>[3x]GPGGAERPTLPIPDLLTTDARNRI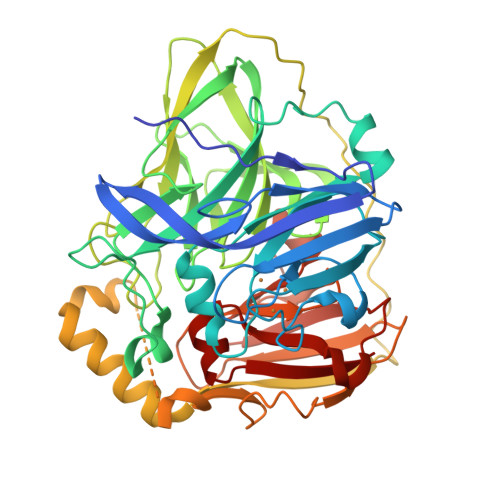QLTIGAGQSTFGGKTATTWGYNGNLLGPAVKLQRGKAVTVDIYNQLTEETTLHWHGLEVPGEVDGGPQGIIPPGGKRSVTLNVDQPAATCWFHPHQHGKTGRQVAMGLAGLVVIEDDEILKLMLPKQWGIDDVPVIVQDKKFSADGQIDYQLDVMTAAVGWFGDTLLTNGAIYPQHAAPRGWLRLRLLNGCNARSLNFATSDNRPLYVIASDGGLLPEPVKVSELPVLMGERFEVLVEVNDNKPFDLVTLPVSQMGMAIAPFDKPHPVMRIQPIAISASGALPDTLSSLPALPSLEGLTVRKLQLSMDPMLDMMGMQMLMEKYGDQAMAGMDHSQMMGHMGHGNMNHMNHGGKFDFHHANKINGQAFDMNKPMFAAAKGQYERWVISGVGDMMLHPFHIHGTQFRILSENGKPPAAHRAGWKDTVKVEGNVSEVLVKFNHDAPKEHAYMAHCHLLEHEDTGMMLGFTV9-(6-DEOXY-BETA-D-ALLOFURANOSYL)-6-METHYLPURINE | C12 H16 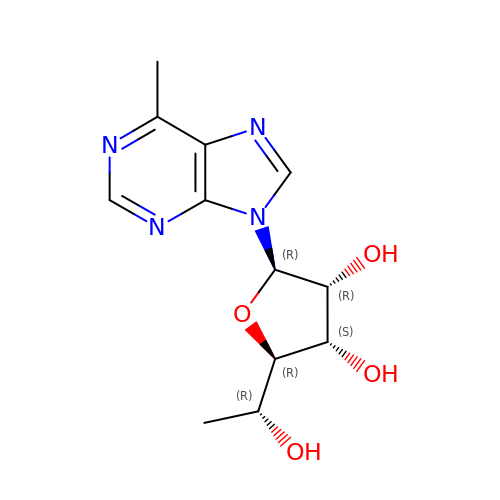N4 O4 | XJZDIUOABWMPLZ-FHQKJXBVSA-N> LVHVASVEKGRSYEDFQKVYNAIALKLREDDEYDNYIGYGPVLVALAWHISGTWDKHDNTGGSYGGTYRFKKEFNDPSNAGLQNGFKFLEPIHKEFPWISSGDLFSLGGVTAVQEMQGPKIPWRCGRVDTPEDTTPDNGRLPDADKDAGYVRTFFQRLNMNDREVVALMGAHALGKTHLKNSGYEGPWGAANNVFTNEFYLNLLNEDWKLEKNDANNEQWDSKSG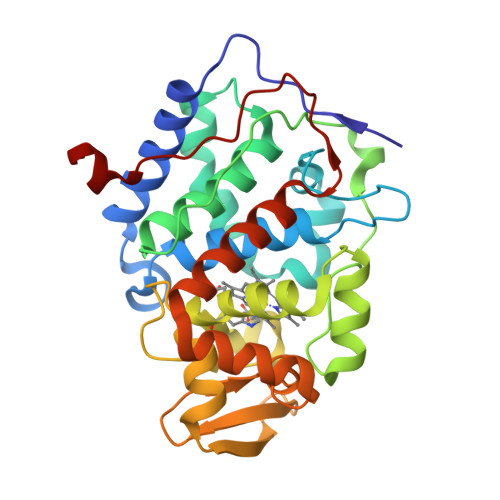YMMLPTDYSLIQDPKYLSIVKEYANDQDKFFKDFSKAFEKLLENGITFPKDAPSPFIFKTLEEQGL>[2x]MTVVSAFLVPGTPLPQLKPEVPSWGQLAAATERAGKALAASRPDVVLVYSTQWLAVLDQQWLTRPRSEGVHVDENWYEFGDLAYDIRADTALAEACVTSSPLHGVHA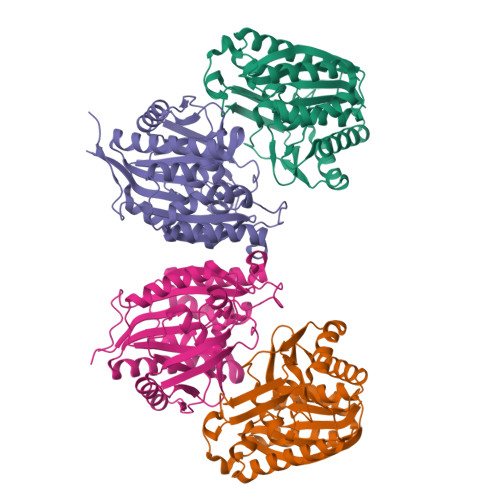RGVNYDGFPIDTGTITACTLMGIGTDAFPLVVGSNNLYHSGEITEKLAALAVDCAKDQNKRVAVVGVGGLSGSLFREEIDPREDRIANEEDDKWNRRVLKLIEAGDVSALREAMPVYAKEARVDMGFKHLHWILGALKGKFSGANVLGYGPSYGSGAAVIEFRL;>[2x]MQGEIIAGFLAPHPPHLVYGENPPQNEPRSQGGWEVLRWAYERARERLDAMKPDVLLVHSPHWITSVGHHFLGVPELSGKSVDPIFPNVFRYDFSLNVDVELAEACAEEGRKAGLVTKMMRNPKFRVDYGTITTLHLIRPQWDIPVVGISANNSPYYLNTKEGMSEMDVLGKATREAIRKTGRKAVLLASNTLSHWHFHEEPTIPEDMSKEYPATMAGYQWDIRMIELMRQGKTSEVFKLLPQFIDEAFAEVKSGAFTWMHAAMQYPELAAELFGYGTVIGTGNAVMEWDLRKAGLSMLGAADQKQRSAAVA>GIASFHPSPWGDYFLKYVPCDQVTQAKMEDEVKKVEEDVKKELRKLAKAVGKPLELLNFIDVVERLGVGYRLEQEIEDLVQAIFDNDKFGVDEFDLYHTSLWFRLLRQHGFHVSCDVFGKFKGRNGRFKDSLASDVKGILGLYEASHVRTHGDDTLDEALVFTTTHLKAVVTNQPNHPLVPQVTHALMQPYHKGMPRLESRHFIAFYEKDPYHDKTLLKFGKLDFNLVQALHKKELKDLSRWWKDLDMHAKMPFPSRDRVPEGYFWTLGPFYEPQFALCRKFFLQVFKVTSIVDDIYDAYGTIDELTAFTKAAERWDRSCLDELPEYMKVSYASLIDTFEEFERDLAPQGRSWSVKYAREEMIQMCRVYYQEAKWCHEKYSPTCDEYLEKASIVSFGYNLGTVVCFLGMGDVATKEAFEWARGNPKVVRAAGIIGRLMDDIGSHHFEQGRDHVPSAVECYIRQHGVDEVTAQRELGKRVESSWKDINEMML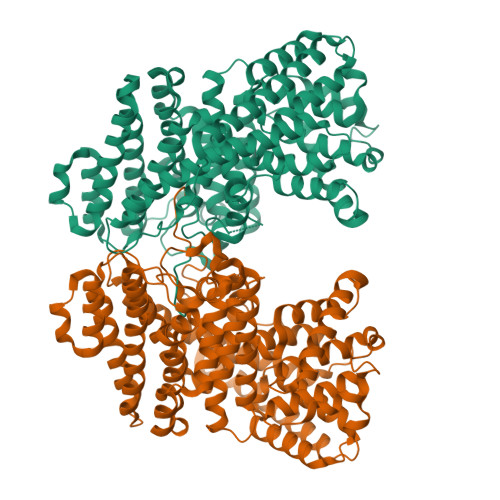KPYMMPKPLLTRILNECRIVDVIYKGEDSYTFSNTTMKKNISHILTDPIPI[2x]> MRAVRLVEIGKPLSLQEIGVPKPKGPQVLIKVEAAGVCHSDVHMRQGRFGNLRIVEDLGVKLPVTLGHEIAGKIEEVGDEVVGYSKGDLVAVNPWQGEGNCYYCRIGEEHLCDSPRWLGINFDGAYAEYVIVPHYKYMYKLRRLNAVEAAPLTCSGITTYRAVRKASLDPTKTLLVVGAGGGLGTMAVQIAKAV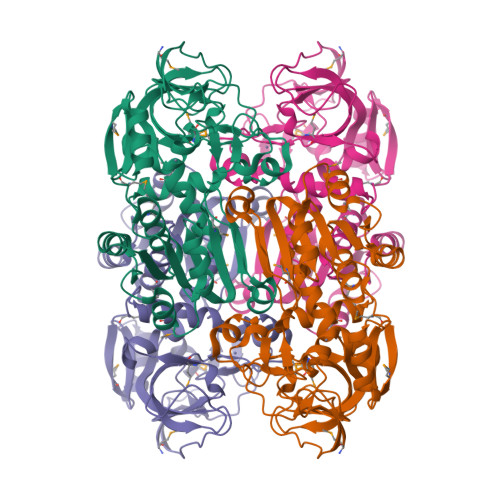SGATIIGVDVREEAVEAAKRAGADYVINASMQDPLAEIRRITESKGVDAVIDLNNSEKTLSVYPKALAKQGKYVMVGLFGADLHYHAPLITLSEIQFVGSLVGNQSDFLGIMRLAEAGKVKPMITKTMKLEEANEAIDNLENFKAIGRQVLIP>MKKGSANEDMPVERILEAELAVEPKTETYVEANMGLNPSSPNDPVTNICQAADKQLFTLVEWAKRIPHFSELPLDDQVILLRAGWNELLIASFSHRSIAVKDGILLATGLHVHRNSAHSAGVGAIFDRVLTELVSKMRDMQMDKTELGCLRAIVLFNPDSKGLSNPAEVEALREKVYASLEAYCKHKYPEQPGRFAKLLLRLPALRSIGLKCLEHLFFFKLIGDTPIDTFLMEMLEAPHQMT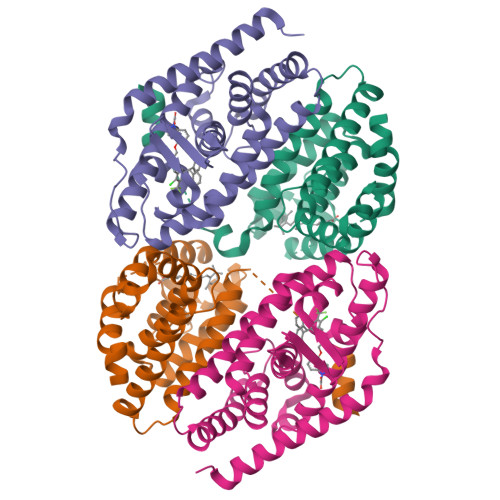[2x];>[2x]MRGSHHHHHHGMASLVPRGSVLPQLSPEQLGMIEKLVAAQQQCNRRSFSDRLRVTPWPIAPDPQSREARQQRFAHFTELAIVSVQEIVDFAKQLPGFLQLSREDQIALLKTSAIEVMLLETSRRYNPGSESITFLKDFSYNREDFAKAGLQVEFINPIFEFSRAMNELQLNDAEFALLIAISIFSADRPNVQDQLQVERLQHTYVEALHAYVSINHPHDPLMFPRMLMKLVSLRTLSSVHSEQVFALRLQDKKLPPLLSEIWDVHE>MQLYSFFNSSTSYRVRIALALKGLDYQVVPVNLRQGEQLRPADRQRNPMGALPTLVDADGRRFSQSLAIIDYLDAVQPEPRLIPLDPLHRAQALELALLVACDIHPLNNVRVLKYLTQVLGIDAEDRQRWYAHWVAEGLAAAETLLNRHRRGAFFAGAAAGIVECCLVPQLANARRMGCDLAPYPALLELEGRCLALEAF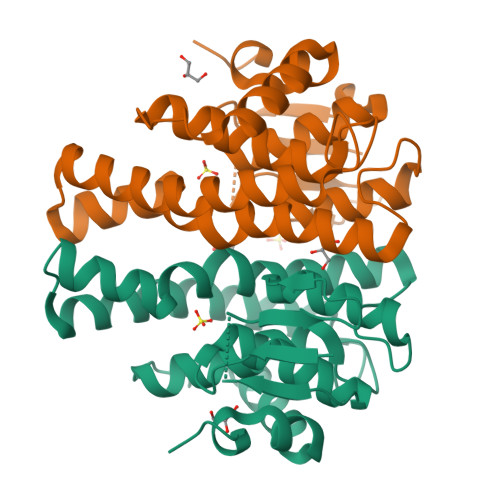QRASPERQPDYLPDLEHHHHHH[2x]>[36x]MGNRGMEDLIPLVNRLQDAFSAIGQNADLDLPQIAVVGGQSAGKSSVLENFVGRDFLPRGSGIVTRRPLVLQLVNATTEYAEFLHCKGKKFTDFEEVRLEIEAETDRVTGTNKGISPVPINLRVYSPHVLNLTLVDLPGMTKVPVGDQPPDIEFQIRDMLMQFVTKENCLILAVSPANSDLANSDALKVAKEVDPQGQRTIGVITKLDLMDEGTDARDVLENKLLPLRRGYIGVVNRSQKDIDGKKDITAALAAERKFFLSHPSYRHLADRMGTPYLQKVLNQQLTNHIRDTLPGLRNKLQSQLLSIEKEVEEYKNFRPDDPARKTKALLQMVQQFAVDFEKRIEGSGDQIDTYELSGGARINRIFHERFPFELVKMEFDEKELRREISYAIKNIHGIRTGLFTPDMAFETIVKKQVKKIREPCLKCVDMVISELISTVRQCTKKLQQYPRLREEMERIVTTHIREREGRTKEQVMLLIDIELAYMNTNHEDFIGFANAQQRSNQMNKKKTSGNQDEILVIRKGWLTINNIGIMKGGSKEYWFVLTAENLSWYKDDEEKEKKYMLSVDNLKLRDVEKGFMSSKHIFALFNTEQRNVYKDYRQLELACETQEEVDSWKASFLRAGVYPERVGDKEKASETEENGSDSFMHSMDPQLERQVETIRNLVDSYMAIVNKTVRDLMPKTIMHLMINNTKEFIFSELLANLYSCGDQNTLMEESAEQAQRRDEMLRMYHALKEALSIIGNINTTTVSTPMPPPVDDSWLQVQSVPAGRRSPTSSPTPQRRAPAVPPARPGSRGPAPGPPPAGSALGGAPPVPSRPGASPDPFGPPPQVPSRPNRAPPGVPSRSGQASPSRPESPRPPFDL

Dynamin (isoforms 1, 2, and 3) is the founding member of a ubiquitous superfamily of large GTPases and is best known for its role in catalyzing membrane scission of cargo-loaded vesicles during endocytosis. Dynamin molecules are recruited to the neck of budding vesicles to assemble into a helical collar and to constrict the underlying membrane. Two hinges are present; Hinge 1 connects the BSE and the Stalk whereas Hinge 2 connects the BSE and the G domain. Various cryoEM reconstructions confirmed that a GG dimer interface forms between two dynamin monomers in helical configurations, and the three conserved Stalk interfaces are vital for dynamin to polymerize into filaments.

Here, we report the structure of a two-start dynamin helix at 3.74 Å resolution. The MBP tagged Dyn1ΔPRD self-assembles into long and straight two-start filaments in the presence of GMP-PCP in the absence of lipid template, same as the untagged Dyn1ΔPRD. It shows a two-start helix with a rise of 13.58 Å and a twist of 24.43°. The three dynamin domains are radially distributed, with the G domain making up the outer surface layer, the BSE in the short middle layer, connecting the G domain and the inner Stalk domain layer, which forms an extended oligomer. The two-start helix comprises of two strands, which are joined by the conserved GG dimeric interfaces contributed by the GTPase domains of the two opposing strands. The density for the bound GMP-PCP nucleotide is clearly discernible (inset). Neither is their density for the PH domain when reconstructions were carried out with or without applying helical symmetry. The two monomers of the GG dimer share the same overall architecture but are not symmetrical, consistent with the GG dimer in the one-start helix12. In comparison with the one-start GG dimer, there is about 3° rotation around Hinge 1 which brings the terminals of the two Stalk domains closer by 8 Å in the two-start GG dimer. Furthermore, the Stalk interface 2 and interface 3 serve as fulcrum points to allow small relative rotations of the Stalk domains, while preserving interface 1 accordingly.>[2x]PPNLTGYYRFVSQKNMEDYLQALNISLAVRKIALLLKPDKEIEHQGNHMTVRTLSTFRN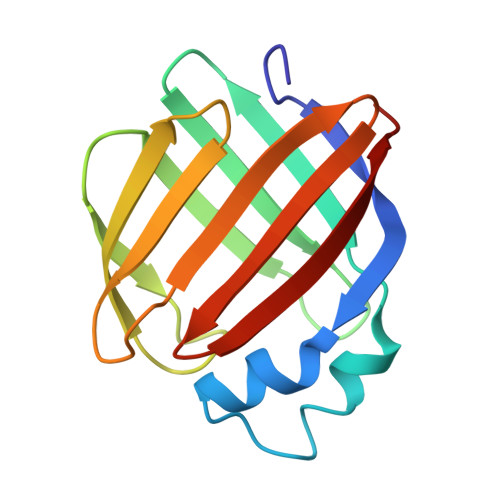YTVQFDVGVEFEEDLRSVDGRKCQTIVTWEEEHLVCVQKGEVPNRGWRHWLEGEMLYLELTARDAVCEQVFRKVH> GSSPKAVALYSFAGEESGDLPFRKGDVITILKKSDSQ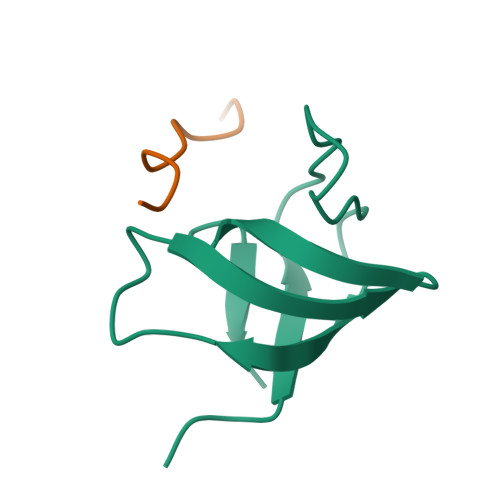NDWWTGRVNGREGIFPANYVELV;> EGPPPAMPARPT> MKAQGETEESEKLSKMSSLLERLHAKFNQNRPWSETIKLVRQVMEKRVVMSSGGHQHLVSCLETLQKALKVTSLPAMTDRLESIARQNGLGSHLSASGTECYITSDMFYVEVQLDPAGQLCDVKVAHHGENPVSCPELVQQLREKNFDEFSKHLKGLVNLYNLPGDNKLKTKMYLALQSLEQDLSKMAIMYWKATNAGPLDKILHGSVGYLTPRSGGHLMNLKYYVSPSDLLDDKTASPIILHENNVSRSLGMNASVTIEGTSAVYKLPIAPLIMGSHPVDNKWTPSFSSITSANSVDLPACFFLKFPQPIPVSRAFVQKLQNCTGIPLFETQPTYAPLYELITQFELSKDPDPIPLNHNMRFYAALPGQQHCYFLNKDAPLPDGRSLQGTLVSKITFQHPGRVPLILNLIRHQVAYNTLIGSCVKRTILKEDSPGLLQFEVCPLSESRFSVSFQHPVNDSLVCVVMDVQDSTHVSCKLYKGLSDALICTDDFIAKVVQRCMSIPVTMRAIRRKAETIQADTPALSLIAETVEDMVKKNLPPASSPGYGMTTGNNPMSGTTTPTNTFPGGPITTLFNMSMSIKDRHESVGHGEDFSKVSQNPILTSLLQITGNGGSTIGSSPTPPHHTPPPVSSMAGNTKNHPMLMNLLKDNPAQDFSTLYGSSPLERQNSSSGSPRMEICSGSNKTKKKKSSRLPPEKPKHQTEDDFQRELFSMDVDSQNPIFDVNMTADTLDTPHITPAPSQCSTPPTTYPQPVPHPQPSIQRMVRLSSSDSIGPDVTDILSDIAEEASKLPSTSDDCPAIGTPLRDSSSSGHSQSTLFDSDVFQTNNNENPYTDPADLIADAAGSPSSDSPTNHFFHDGVDFNPDLLNSQSQSGFGEEYFDESSQSGDNDDFKGFASQALNTLGVPMLGGDNGETKFKGNNQADTVDFSIISVAGKALAPADLMEHHSGSQGPLLTTGDLGKEKTQKRVKEGNGTSNSTLSGPGLDSKPGKRSRTPSNDGKSKDKPPKRKKADTEGKSPSHSSSNR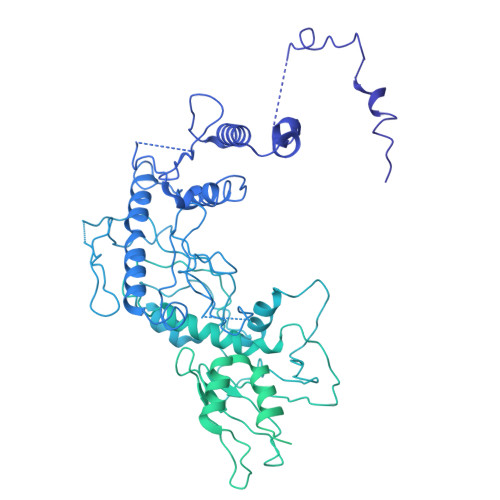PFTPPTSTGGSKSPGSAGRSQTPPGVATPPIPKITIQIPKGTVMVGKPSSHSQYTSSGSVSSSGSKSHHSHSSSSSSSASTSGKMKSSKSEGSSSSKLSSSMYSSQGSSGSSQSKNSSQSGGKPGSSPITKHGLSSGSSSTKMKPQGKPSSLMNPSLSKPNISPSHSRPPGGSDKLASPMKPVPGTPPSSKAKSPISSGSGGSHMSGTSSSSGMKSSSGLGSSGSLSQKTPPSSNSCTASSSSFSSSGSSMSSSQNQHGSSKGKSPSRNKKPSLTAVIDKLKHGVVTSGPGGEDPLDGQMGVSTNSSSHPMSSKHNMSGGEFQGKREKSDKDKSKVSTSGSSVDSSKKTSESKNVGSTGVAKIIISKHDGGSPSIKAKVTLQKPGESSGEGLRPQMASSKNYGSPLISGSTPKHERGSPSHSKSPAYTPQNLDSESESGSSIAEKSYQNSPSSDDGIRPLPEYSTEKHKKHKKEKKKVKDKDRDRDRDKDRDKKKSHSIKPESWSKSPISSDQSLSMTSNTILSADRPSRLSPDFMIGEEDDDLMDVALIGN>MAKKTGAKYPKSLLSLPLVGSLPFLPRHGHMHNYFFKLQKKYGPIYSVRMGTKTTVIVGHHQLAKEVLIKKGKDFSGRPQMATLDIASNNRKGIAFADSGAHWQLHRRLAMATFALFKDGDQKLEKIICQEISTLCDMLATHNGQSIDISFPVFVAVTNVISLICFNTSYKNGDPELNVIQNYNEGIIDNLSKDSLVDLVPWLKIFPNKTLEKLKSHVKIRNDLLNKILENYKEKFRSDSITNMLDTLMQAKMNSDNGNAGPDQDSELLSDNHILTTIGDIFGAGVETTTSVVKWTLAFLLHNPQVKKKLYEEIDQNVGFSRTPTISDRNRLLLLEATIREVLRLRPVAPMLIPHKANVDSSIGEFAVDKGTEVIINLWALHHNEKEWHQPDQFMPERFLNPAGTQLISPSVSYLPFGAGPRSCIGEILARQELFLIMAWLLQRFDLEVPDDGQLPSLEGIPKVVFLIDSFKVKIKVRQAWREAQAEGS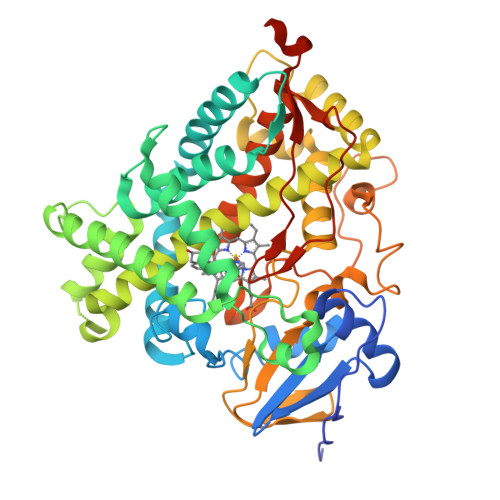THHHH[2x]5-bromo-3-(pyrrolidin-1-ylsulfonyl)-1H-indole-2-carboxamide 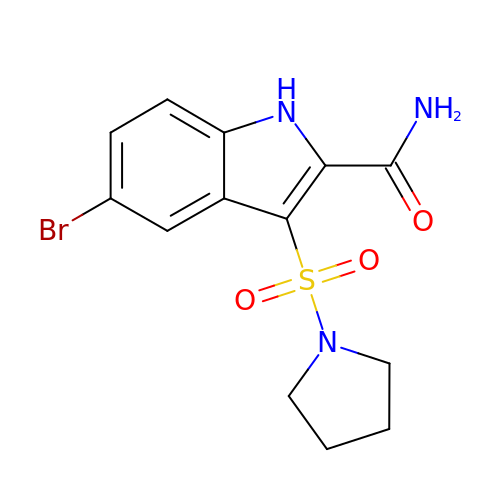| C13 H14 Br N3 O3 S | FEPUPYVRZUWCQB-UHFFFAOYSA-N>[2x]QQRFPQRYVMLAIVADHGMVTKYSGNSSAITTRVHQMVSHVTEMYSPLNIATTLSLLRIWSSKDLITVQSDSSVTLGSFGDWRKVVLLSQQAHDCA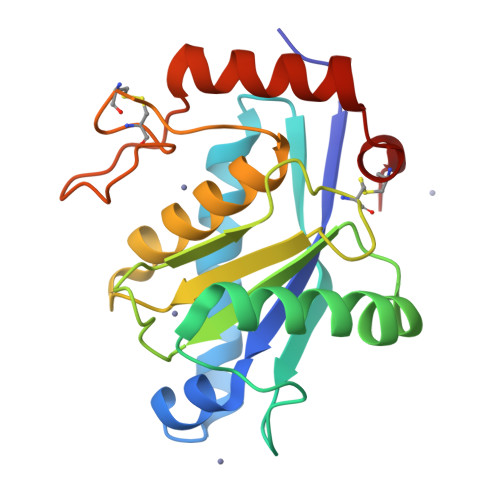FLNTATALDDSTIGLAYSNGMCDPKFSVGLVQDHSSNVFMVAVTMTHELGHNLGMAHDEAGGCACSSCIMSPAASSGPSKLFSDCSKDDYQTFLTNTNPQCILNAP>MFPKALGYVTGDMKELANQLKDKPVVLQFIDWILRGISQVVFVNNPVSGILILVGLLVQNPWWALTGWLGTVVSTLMALLLSQDRSLIASGLYGYNATLVGVLMAVFSDKGDYFWWLLLPVCAMSMTCPIFSSALNSVLSKWDLPVFTLPFNMALSMYLSATGHYNPFFPAKLVIPITTAPQISWSDLSALELLKSIPVGVGQIYGCDNPWTGGIFLGAILLSSPLMCLHAAIGSLLGIAAGLSLSAPFENIYFGLWGFNSSLACIAMGGMFMALTWQTHLLALGCALFTAYLGVGMANFMAEVGLPACTWPFCLATLLFLIMTTKNSNIYKMPLSKVTYPEENRIFYLQAKKRMVESPLAENLYFQ[3x]

While the initial excretion occurs through diffusion across the membrane, the subsequent reabsorption is mediated by urea transporters UT-A (HsUT-A; SLC14A2) and UT-B (HsUT-B; SLC14A1) which are differentially expressed in specific renal tubule compartments. The overall structures of HsUT-A and HsUT-B are similar to each other and to BtUT-B and DvUT, showing the trimeric arrangement with 10 TM helices and two pore (P) helices per subunit. In both structures, each subunit hosts a channel-like pore for urea transport and the channels are in the open state with approximately 2 to 3 Å in diameter at constriction formed by V69, T177, L292, and F342.

UTBinh-14 is a highly selective inhibitor for UT-B, with over a thousand-fold selectivity over UT-A. Owing to such properties, it has been used as a chemical probe to study physiological roles of UT-B and is an attractive lead molecule for a drug discovery program. Hypothesizing that this could be due to either the combination of low solubility and low affinity of UTBinh-14 or its low stability, we changed our structure determination technique to cryo-EM. This resulted in a refined ESP map with 2.6 Å nominal resolution, showing little conformational change and revealing UTBinh-14 blocking the channel on the extracellular side. UTBinh-14 fits well into this extracellular pocket, with its 2-thienyl group directly blocking the pore entry. The inhibitor forms hydrophilic interactions with the side chain of Q232 and the backbone carbonyl of A337 of HsUT-B, and its 4-ethylbenzene group sits in a hydrophobic pocket formed by W286, F288, G323, and A327. An interesting feature of the binding mode of UTBinh-14 is its 2-thienyl group at the channel pore entry. This group is in close proximity to C338 with its sulfur atom facing toward the residue, and this has forced the side chain of C338 to rotate away (with respect to the apo state) from the pore entry due to steric clash. Therefore, it is possible that the inhibitor could form a covalent bond with UT-B at C338 if the 2-thienyl group was replaced with a thiol group. Our cryo-EM map of UTBinh-14–bound HsUT-B shows a small molecule feature on the intracellular side of the channel pore. Real-space refinement with Phenix estimates its occupancy at 0.38, and the incomplete occupancy by UTBinh-14 suggests low binding affinity at this site compared to the extracellular one.> AKGTTCQKAIVNWEAANPGKNPSEAEEIKLIFQIPPIEKMDGPVLNTLTKCKKLSLSSNSIDKMISLNMLRNLEILSLSRNVIKKISGLEDIGGTLRQLWLSYNFIEKLDGLNNCSVLQTLYIGNNRIKN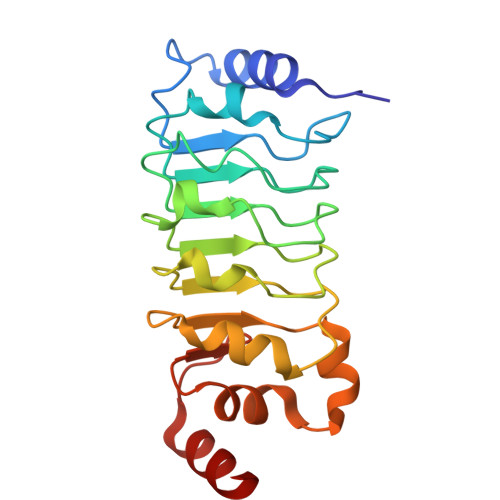WEELDKLKDLPELENVLFYGNPIYEQVKEDPKLIVLKKLPTLKNVDGMIIDDSVLEKVKQIA> GPHMKSPSAQELKEQGNRLFVGRKYPEAAACYGRAITRNPLVAVYYTNRALCYLKMQQPEQALADCRRALELDGQSVKAHFFLGQCQLEMESYDEAIANLQRAYSLAKEQRLNF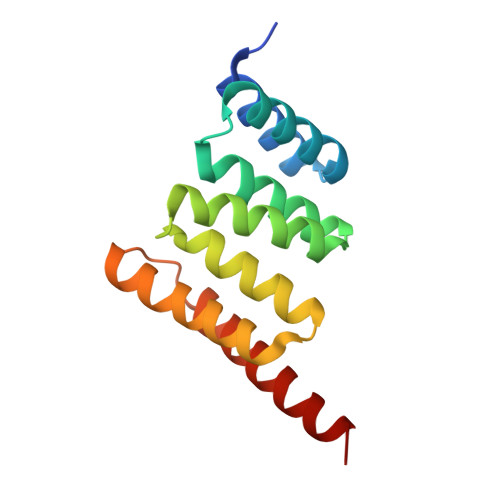GDDIPSALRIAKKKRWNSIEERR>[2x]MQHLDIAELVRSALEVSGCDPSLIGGIDSHSTIVLDLFALPSICISVKDDDVWIWAQLGADSMVVLQQRAYEILMTIMEGCHFARGGQLLLGEQNGELTLKALVHPDFLSDGEKFSTALNGFYNYLEVFSRSLMR;> QATNLAANLSAVRESATATLSGEIKGPQLEDFPALIKQASLDALFKCGKDAEALKEVFTNSNNVAGKKAIME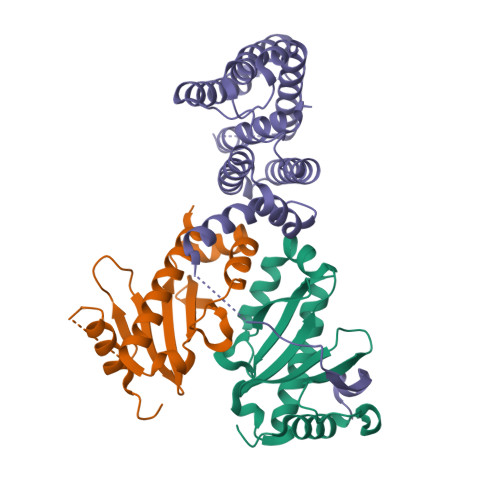FAGLFRSALNATSDSPEAKTLLMKVGAEYTAQIIKDGLKEKSAFGPWLPETKKAEAKLENLEKQLLDIIKNNTGGELSKLSTNLVMQEVMPYIASCIEHNFGCTLDPLTRSNLTHLVDKAAAKAVEALDMCHQKLTQEQGTSVGREARHLEMQTLIPLLLRNVFAQIP> MNTIFSARIMKRLALTTALCTAFISAAHADDLNIKTMIPGVPQIDAESYILIDYNSGKVLAEQNADVRRDPASLTKMMTSYVIGQAMKAGKFKETDLVTIGNDAWATGNPVFKGSSLMFLKPGMQVPVSQLIRGINLQSGNDACVAMADFAAGSQDAFVGLMNSYVNALGLKNTHFQTVHGLDADGQYSSARDMALIGQALIRDVPNEYSIYKEKEFTFNGIRQLNRNGLLWDNSLNVDGIKTGHTDKAGYNLVASATEGQMRLISAVMGGRTFKGREAESKKLLTWGFRFFETVNPLKVGKEFASEPVWFGDSDRASLGVDKDVYLTIPRGRMKDLKASYVLNSSELHAPLQKNQVVGTINFQLDGKTIEQRPLVVLQEIPEGNFFGKIIDYIKLMFHHWFG

Despite the success of beta-lactam antibiotics in the clinic, it has recently been shown that an alternate crosslinking mechanism can lead to the bypass of PBP mediated D,D-transpeptidation. The L,D-transpeptidase YcbB (alternately named LdtD), with remarkably few additional accessory factors, is able to undertake this recovery of PG crosslinking function, even in the presence of many clinically used beta-lactam antibiotics. As with D,D-crosslinked PG, the bypass pathway initiates with GTase catalyzed polymerisation of PG; the resultant growing product strand is acted upon by PBP5 which catalyses a carboxypeptidase reaction targeting removal of the terminal D-Ala5 resulting in a donor glycan-tetrapeptide substrate for YcbB. In the last step of the bypass pathway, YcbB catalyses L,D-transpeptidation using this tetrapeptide-containing donor to form a DAP3donor-DAP3acceptor crosslink.

In addition, we report in parallel, the structure of a PBP5-meropenem acyl enzyme complex in order to completely describe the molecular interactions which facilitate meropenem inhibition of the YcbB and PBP5 partners. A 2.2 Å resolution structure of PBP5 acylated with meropenem was also solved with very well ordered density for the covalently bound meropenem. Relative to previously published PBP5 structures, we were able to trace additional residues at the C-terminus of PBP5 (387–397; likely afforded by the differential packing with a neighbouring molecule in our unique crystal lattice). Regardless, the conserved binding mode of the ligands between the PBP5-meropenem structure and the PBP5-imipenem structure (PDB ID 3MZF24) indicates similar modes of enzyme acylation and binding. Meropenem binds PBP5 in a typical PBP fashion using the conserved SXXK, SXN, and KTG active site sequence motifs common to this broad class of activated serine carboxypeptidases. The meropenem is acylated at C7 by the Ser73 side chain hydroxyl of the SXXK motif (the proximal Lys76 of the motif playing the general base role) and stabilised through an extensive hydrogen bond and electrostatic network. The carbonyl oxygen on C7 of meropenem occupies the enzyme oxyanion hole comprised of main chain nitrogens at position 73 and 245, forming strong hydrogen bonds that polarize and stabilize the carbonyl during acylation and formation of oxycarbanion intermediates. The side chain hydroxyl of Ser 139 of the SXN motif resides adjacent to the leaving group nitrogen of meropenem, the likely source for protonation of that moiety to promote acylation. The Asn141 side chain amide of the SXN motif hydrogen bonds with the 1-hydroxyethyl group on C6 of meropenem, while the Thr243 side chain hydroxyl of the KTG motif forms bidentate hydrogen bonds to the carboxylic acid group of meropenem (C3). The latter is further stabilized by longer range electrostatic interactions with the side chain amido of Lys242 of the motif as well as the guanidinium group of Arg277.>MTQTTQSPALIASQSSWRCVQAHDREGWLALMADDVVIEDPIGKSVTNPDGSGIKGKEAVGAFFDTHIAANRLTVTCEETFPSSSPDEIA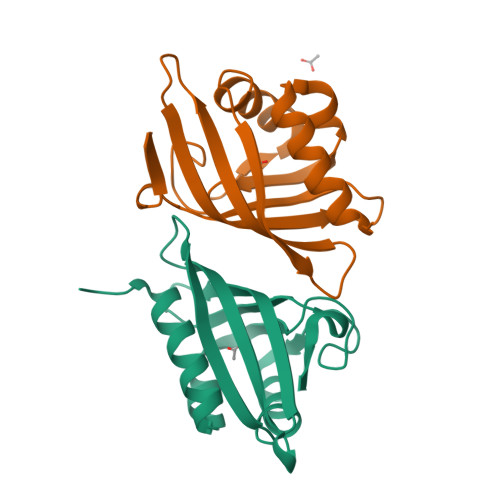HILVLHSEFDGGFTSEVRGVFTYRVNKAGLITNMRGYWNLDMMTFGNQE[4x]> MGSSHHHHHHSSGRENLYFQGHMVSLDKAVIARLRKGGEEFEVLVDPYLARDLKEGKEVNFEDLLAAEEVFKDAKKGERASVDELRKIFGTDDVFEIARKIILEGEVQITAEQ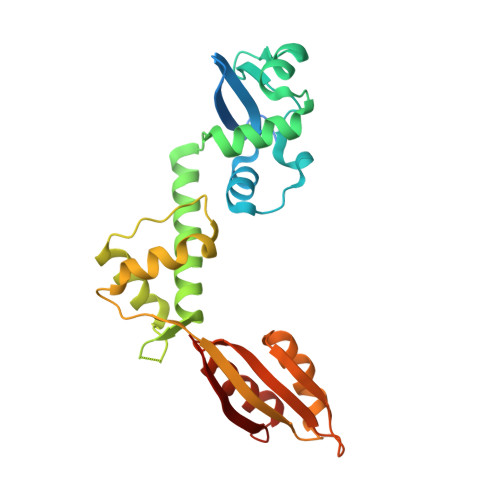RREMLEAKRKQIINFISRNTIDPRTNAPHPPSRIERALEEAKVHIDIFKSVEAQVKDIVKALKPILPLKFEEMEIAIKIPPEHTGRAISALYNFGGVTREEWQRDGSWICVMRIPSGMYGDLMDLLGKVAKGEALTKVLRRIG In the initial step, phosphatidylinositol-phosphate (PIP) synthases generate PIP using L-myo-inositol-1-phosphate (inositol phosphate) as the acceptor alcohol and CDP-DAG as the donor substrate; subsequently, the terminal phosphate is removed by an as-yet-unidentified phosphatase to yield PI4. All (class I) CDP-APs are integral membrane enzymes that catalyse the transfer of a substituted phosphate group from a CDP-linked donor, CDP-DAG for PI and PIP biosynthesis, to an acceptor alcohol to generate a phosphodiester-linked product. We have determined the crystal structures of PIP synthase from Renibacterium salmoninarum, in the apo form and with bound CDP-DAG to 2.5 and 3.6 Å resolution, respectively. RsPIPS adopts a homodimeric architecture similar to those previously observed in Af2299 and AfDIPP synthase, with each protomer possessing six TM helices surrounding a large polar cavity.

Subsequently, we determined the structure of a construct containing the complete RsPIPS sequence (absent the initiating methionine; RsPIPS-FL) in complex with CDP-DAG at 3.6 Å resolution, again by molecular replacement, in this instance using RsPIPS-Δ6N as search model. In contrast, although crystals of RsPIPS-FL only diffracted to lower resolution (3.6 Å), a structure of the complex with CDP-DAG was obtained readily. The structure of the complex of CDP-DAG bound to RsPIPS-FL revealed strong density for CDP, with the nucleotide ring wedged between TMs 2 and 3, and the diphosphate moiety coordinated by a bound magnesium ion that also interacts with conserved aspartate residues of the CDP-AP signature sequence. In all four protomers in the asymmetric unit, density was also observed for the acyl chains of the CDP-DAG, which lie against the TM region in a groove formed by JM1, TM2 and TM5. This groove is entirely absent in the two previous structures of CDP-APs, which have a small, hydrophilic pocket in this location, consistent with their preference for soluble donor moieties such as CDP-glycerol and CDP-inositol. A unique feature of the structure of RsPIPS when compared with Af2299 and AfDIPP synthase is the presence of a hydrophobic crevice between JM1, TM2 and TM5, which in the structure of RsPIPS-FL accommodates the lipid substrate. This groove is directly exposed to the bulk lipid, providing a pathway for lateral diffusion of CDP-DAG into the active site. The nucleotide is wedged between TM2 and TM3 in a pocket, which is also lined by TM1. The CDP interacts with residues from the signature sequence on TM2 and TM3. In addition, D29 and T32, part of a conserved P(D/N)xx(T/S) motif at the start of TM1, form hydrogen bonds with polar substituents of the pyrimidine ring.

>MRLAYVKNHEIYGEKLLGLTLRERIEKTLQRAGFDVRFFDELSLEEAEDYLIILEPVLILERDLLLEGRKILVSDGFTVGYFFGGDFRTVFDGNLQSSIEKYLSLNNLESYEIWAIKLSNDNLKTAEKLLLSSLIGSGSLNKYARGLFAAIFLPIARLLADWGVSPDAVTVVGTLGVMAGALIFYPMGQLFWGTVVITVFVFSDIIDGLMARLLFREGPWGAFLDSYLDRVGDSSVFTGIVIWFFLGGANPTIAILALICLVLSSLVSYSKARAEGLGLTANVGIAERSERLVVVLVATGLVGLGIPSWVLLVVLIVLAIASVVTIFQRVLTVREQAKAWTA[4x]>[2x]RLLEDALIAVRQQTAMMRKFLDTPGKLMDALKCCSTLVSELRTSSLSPKQYYELYMAVFDALRYLSAHLRENHPV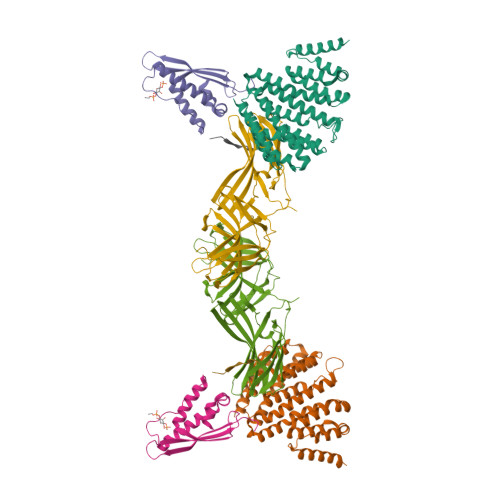NHLADLYELVQYAGNIIPRLYLMITVGTAYMSIDGAPVKELMKDMMDMSRGVQHPVRGLFLRYYLSGQARDYLPTGDSDGPEGNLQDSINFILTNFVEMNKLWVRLQHQGHSRERDLRTQERRELQLLVGSNIVRLSQLVDLPTYRDSILGPLLEQIVQCRDILAQEYLLEVITQVFPDEYHLHTLDQFLGAVSRLNPHVNVKAIVIGMMNRLSDYAERE;>FSTPVDIDIVLADADKRAMVDVKLDKNRREKVPLYMDGESVKGCVTVRPKDGKRLEHTGIKVQFIGTIEMFFDRGNHYEFLSLVQELAAPGELQHPQTFDFNFKNVEKQYESYNGINVKLRYFVRVTVSRRMADVIREKDIWVYSYRIPPELNSSIKMDVGIEDCLHIEFEYSKSKYHLKDVIVGRIYFLLVRLKIKHMELSIIRRETTGVAPNQYNESETLVRFEIMDGSPSRGETIPIRLFLGGFDLTPTFRDVNKKFSTRYYLSLVLIDEDARRYFKQSEIILYRQPPE[2x];>[2x]PPENFLEIEVRNPQTHGVGRHMYTDYEIVCRTNIPAFKLRQSSVRRRYSDFEYFRDILERESARVTIPPLPGKVFTNRFSDEVIENRRAGLEKFLKIVVGHPLLQTGSKVLAAFVQ;>QPELYLLNTM[2x]> PIELPPTYITPYPEISAGGNGTYRGQDL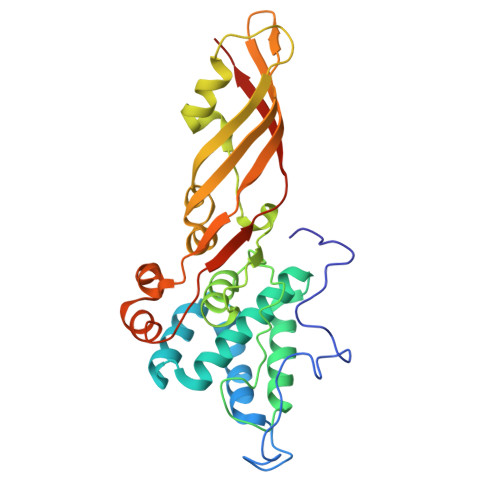SSGQSFPRGMQNPVATVLLLQGDLYCSPNCLATFQDQARRDSFGIQSKVALKTFAAADQREAEGRDLRTAYNEIATDIGRSQQINENIIKYPPGNHVLSGGLMTPFHALAHGMFGLGAPLTFPIQNVGLNVDIRGIPDVMNVIQSARPVGTSSLDVNFAYDVGKDSNASWLTLGNITLRLVGTIDKNASGAWTFSGEIRAFNAVYDANPSNHRGWLGENLTSLLSAVPFTSYSIEIPGSLPVTVSGNLEHHHHHH[1,3-diethyl-2,2-bis(oxidanylidene)-2$l^{6},1,3-benzothiadiazol-5-yl]-(1-methyl-5-oxidanyl-pyrazol-4-yl)methanone 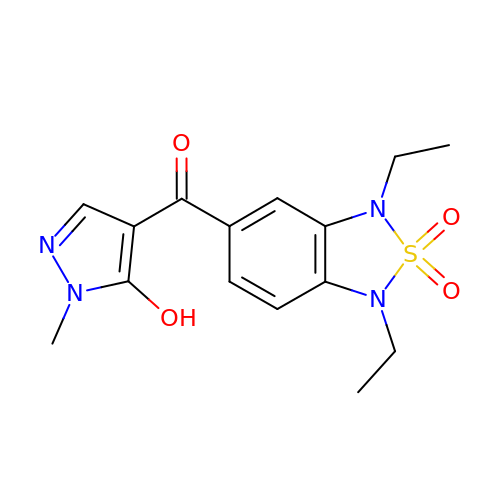| C15 H18 N4 O4 S | QVDQRUFZWCVKJE-UHFFFAOYSA-N> SSADKERLARENHSEIERRRRNKMTAYITELSDMVPTCSALARKPDKLTILRMAVSHMKSLRGTGNTSTDGSYKPSFLTDQELKHLILEAADGFLFIVSCETGRVVYVSDSVTPVLNQPQSEWFGSTLYDQVHPDDVDKLREQLSTSENALTGRVLDLKTGTVKKEGQQSSMRMCMGSRRSFICRMRCGTSSVDPVSMNRLSFLRNRCRNGLGSVKEGEPHFVVVHCTGYIKAWPPAGVSLPDDDPEAGQGSKFCLVAIGRLQVTSSPNCTDMSNICQP;> MYRSTKGASKARRDQINAEIRNLKELLPLAEADKVRLSYLHIMSLACIYTRKGVFFAGGTPLAGPTGLLSAQELEDIVAALPGFLLVFTAEGKLLYLSESVSEHLGHSMVDLVAQGDSIYDIIDPADHLTVRQQLTMPSALDADRLFRCRFNTSKSLRRQSSGNKLVLIRGRFHAHPPGAYWAGNPVFT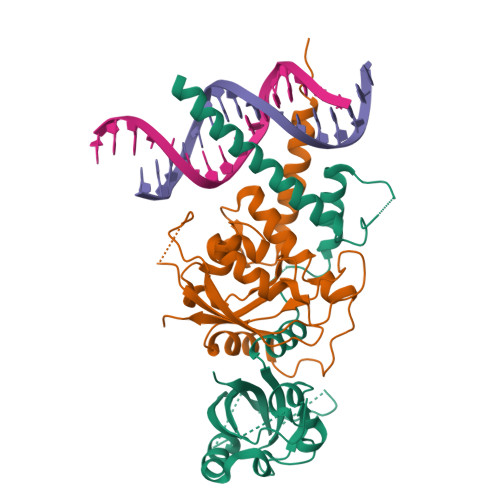AFCAPLEPRPRPGPGPHHHHHH>[6x]GNL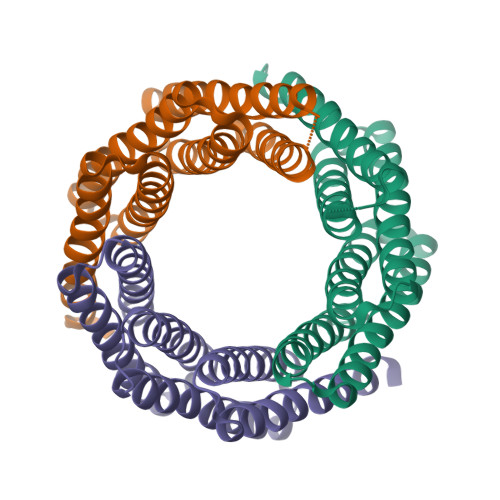ELALKALQILVNAAYVLAEIARDRGNEELLEKAARLAEEAARQAEEIARQARKEGNLELALKALQILVNAAYVLAEIARDRGNEELLEKAARLAEEAARQAEEIARQARKEGNLELALKALQILVNAAYVLAEIARDRGNEELLEKAARLAEEAARQAEEIARQARKEG>[6x]MNAEINPLHAYFKLPNTVSLVAGSSEGETPLNAFDGALLNAGIGNVNLIRIS;>XIMPPEAEIVPLPKLPMGALVPTAYGYIISDVPGETISAAISVAIPK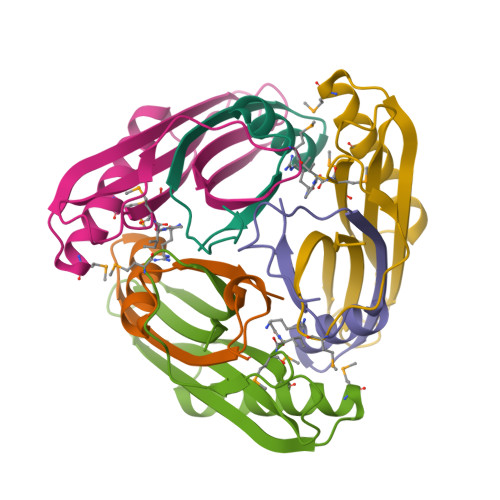DKSLCGLIMEYEGKCSKKEAEKTVREMAKIGFEMRGWELDRIESIAVEHTVEKLGCAFAAAALWYK[6x]> MPSELTPEERSELKNSIAEFHTYQLDPGSCSSLHAQRIHAPPELVWSIVR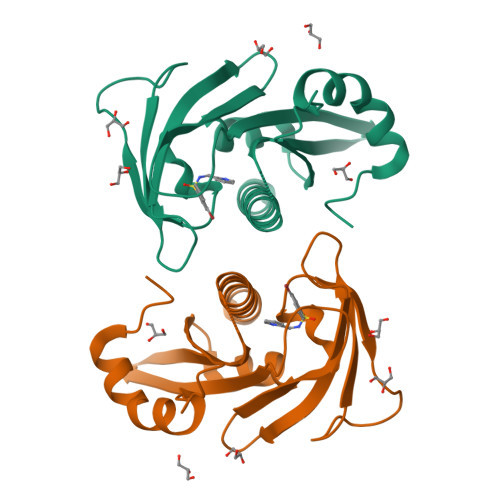RFDKPQTYKHFIKSCSVEQNFEMRVGCTRDVIVISGLPANTSTERLDILDDERRVTGFSIIGGEHRLTNYKSVTTVHRFEKENRIWTVVLESYVVDMPEGNSEDDTRMFADTVVKLNLQKLATVAEAMARN>[2x]GSEHLKNISPIDGRYKKACGELSAFFSEHALIKHRIIVEVRWLLFLNEEELFFEKVTDHSVEVLNQIATNITDSDIARVKAIEEETNHDVKAVEYFVKEKLKNSKREDLLKIKEYVHYLCTSEDINNVAYATCLKACLNDVVIPCLEKIMLKLKDLAVEYSHVPLLSRTHGQPASSTTFGKEMANFYARIHHHVGVIRRVKV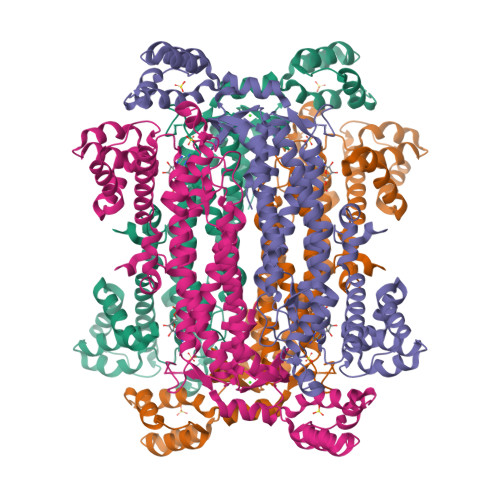CAKFNGAVGNFNAHKVASKDTDWVNTIGLFLKKHFNLTYSIYCTQIQDHDYICELCDGLARANGTLIDLCVDIWLYISNNLLKLKVKEKEVGSSTMPHKVNPIDFENAEGNLHIANAFFKLFSSKLPTSRLQRDLSDSTVLRNIGSSLAYCLIAYKSVLKGLNKIDIDRRNLEEELNQNWSTLAEPIQIVMKRHNYVDAYEELKQFTRGKVIDQKIMQEFIKTKCAFLPQDVVDQLLELTPATYTGYADYLAKNVERLSGERD> GPMATVFRQENVDDYYDTGEELGSGQFAVVKKCREKSTGLQYAAKFIKKRRTKSSRRGVSREDIEREVSILKEIQHPNVITLHEVYENKTDVILILELVAGGELFDFLAEKESLTEEEATEFLKQILNGVYYLHSLQIAHFDLKPENIMLLDRNVPKPRIKI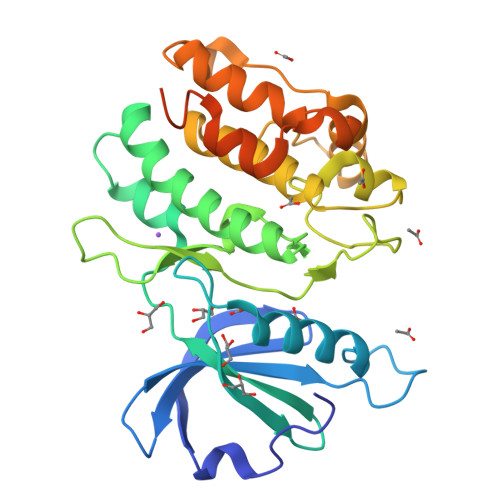IDFGLAHKIDFGNEFKNIFGTPEFVAPEIVNYEPLGLEADMWSIGVITYILLSGASPFLGDTKQETLANVSAVNYEFEDEYFSNTSALAKDFIRRLLVKDPKKRMTIQDSLQHPWIKPKDTQQALSRKAEAVNMEKFKKFAARKKWKQEVR>[2x]MGSSHHHHHHSSGLVPRGSTSEVIEDEKQFYSKAKTYWKQIPPTVDGMLGGYGHISSIDINSSRKFLQRFLREGPNKTGTSCALDCGAGIGRITKRLLLPLFREVDMVDITEDFLVQAKTYLGEEGKRVRNYFCCGLQDFTPEPDSYDVIWIQWVIGHLTDQHLAEFLRRCKGSLRPNGIIV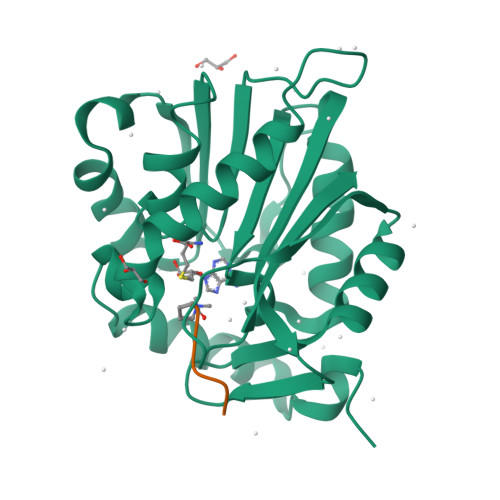IKDNMAQEGVILDDVDSSVCRDLDVVRRIICSAGLSLLAEERQENLPDEIYHVYSFALR;>XPKRIA[2x]>MNPKAVKRENRYANLIPMQEIKSVEQQLYPFDIYNSLRQEAPIRYDESRNCWDVFDYETVKYILKNPSLFSSKRAMEERQESILMMDPPKHTKLRNLVNKAFTPRAIQHLEGHIEEIADYLLDEVSSKEKFDIVEDFAGPLPIIVIAELLGVPIQDRALFKKYSDDLVSGAENNSDEAFAKMMQKRNEGVIFLQGYFKEIIAERQQNKQEDLISLLLEAEIDGEHLTEEEVLGFCILLLVAGNETTTNLITNGVRYMTEDVDVQNEVRRDISLVPNLVEET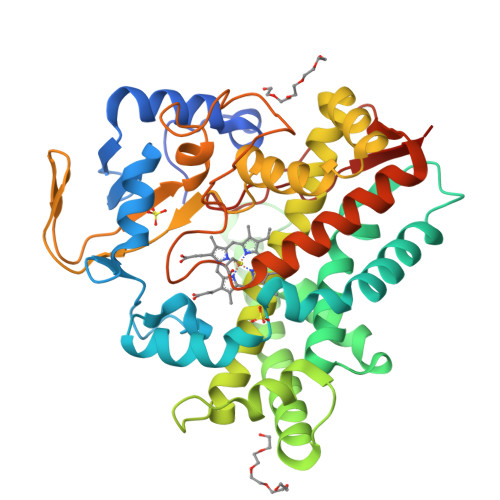LRYYPPIQAIGRIAAEDVELGECKIKRGQQVISWAASANRDSAKFEWPDTFVVHRKTNPHVSFGFGIHFCLGAPLARMEGKIAFTKLLEKGGFSKVQNQSLKPIDSPFVFGVKKYEIAFNNAHHHHHH[4x]> MATQGVFTLPANTRFGVTAFANSSGTQTVNVLV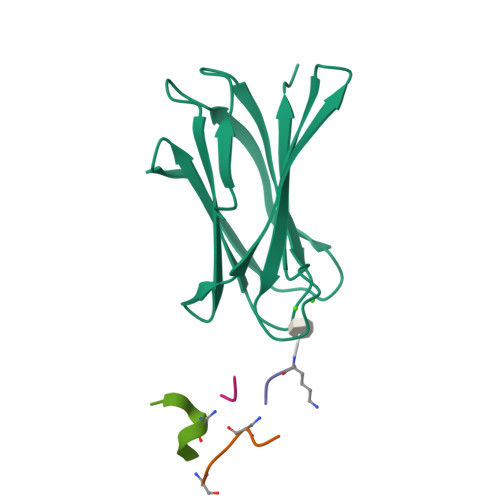NNETAATFSGQSTNNAVIGTQVLNSGSSGKVQVQVSVNGRPSDLVSAQVILTNELNFALVGSEDGTDNDYNDAVVVINWPLG;> KPLAFKA;>[2x]KPL;> KPLAFK> MGDLSCPEGLEELLSAPPPDLGAQRRHGWNPKDCSENIEVKEGG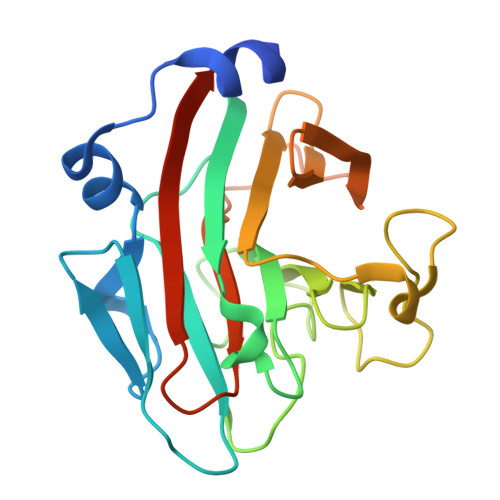LYFERRPVAQSTDGARGKRGYSRGLHAWEISWPLEQRGTHAVVGVATALAPLQTDHYAALLGSNSESWGWDIGRGKLYHQSKGPGAPQYPAGTQGEQLEVPERLLVVLDMEEGTLGYAIGGTYLGPAFRGLKGRTLYPAVSAVWGQCQVRIRYLGERGSHHHHHH> GHHHHHHHHHHSGENLYFQGHMATFISVQLKKTSEVDLAKPLVKFIQQTYPSGGEEQAQYCRAAEELSKLRRAAVGRPLDKHEGALETLLRYYDQICSIEPKFPFSENQICLTFTWKDAFDKGSLFGGSVKLALASLGYEKSCVLFNCAALASQIAAEQNLDNDEGLKIAAKHYQFASGAFLHIKETVLSALSREPTVDISPDTVGTLSLIMLAQAQEVFFLKATR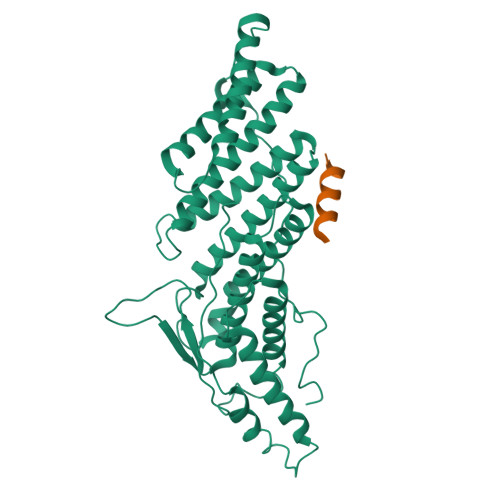DKMKDAIIAKLANQAADYFGDAFKQCQYKDTLPKEVFPVLAAKHCIMQANAEYHQSILAKQQKKFGEEIARLQHAAELIKTVASRYDEYVNVKDFSDKINRALAAAKKDNDFIYHDRVPDLKDLDPIGKATLVKSTPVNVPISQKFTDLFEKMV;> QRAEEEDDDIKQLAAWAT adenosine 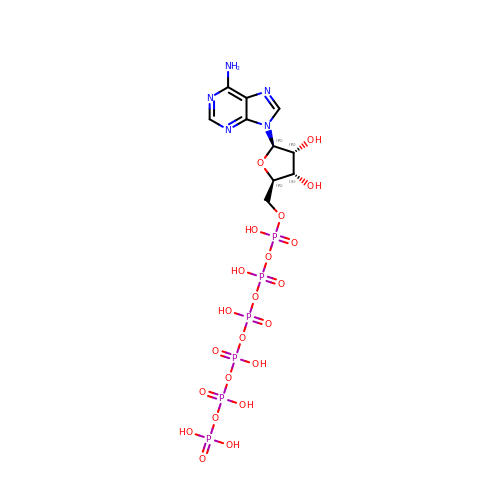5'-hexaphosphate | C10 H19 N5 O22 P6 | MCJDQUICRUJHMC-KQYNXXCUSA-N> GSHMGALKPAKAIVEALLFAAGDEGLSLSQIAAVL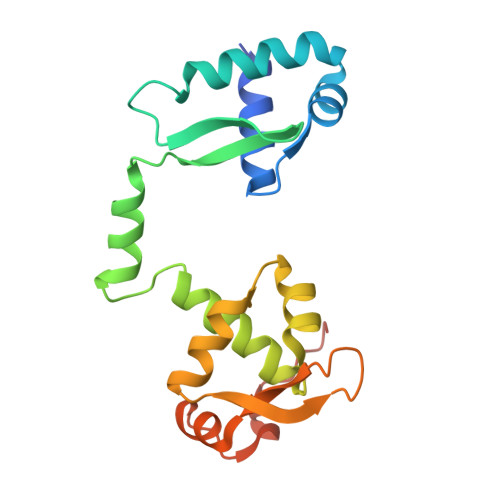EVSELEAKAVIEELQQDCRREERGIQLVELGGVFLLATKKEHAPYLKKLVEAPGASPLSQAALETLAIIAYRQPITRAEIEEIRGVKSDKPLQTLMARALIKEVGRAEGTGRPILYGTTPEFLDYFGLKTLEELPPLPEWADDGESERE>[6x]MKQVTAIIKPFKLDEVRESLAEVGVTGLTVTEVKGFGRQKGHTELY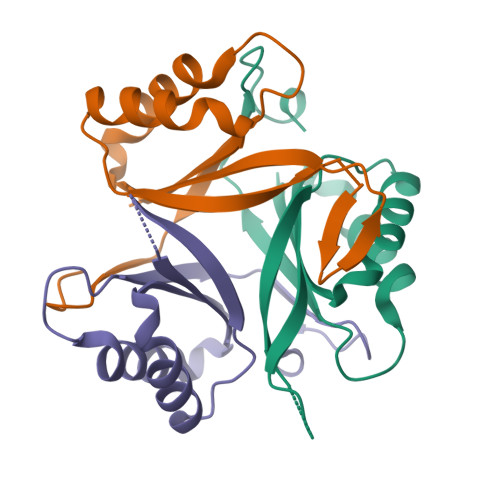RGAEYVVDFLPKVKIEVVVDDKVVEQAVDAIIKAARTGKIGDGKIFVQEVEQVIRIRTGETGPDAV>[2x]MHHH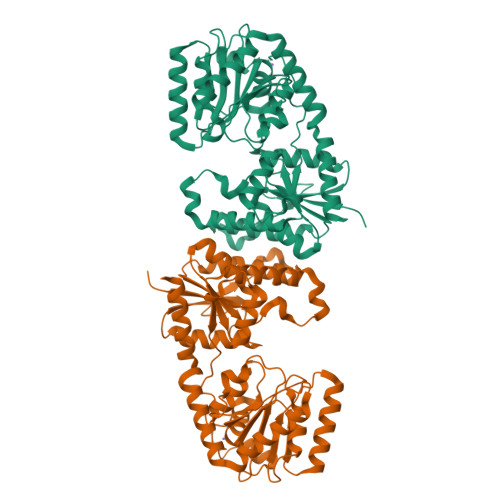HHHENLYFQGMRVAMMTREYPPEVYGGAGVHVTELVAQLRKLCDVDVHCMGAPRDGAYVAHPDPTLRGANAALTMLSADLNMVNNAEAATVVHSHTWYTGLAGHLASLLYGVPHVLTAHSLEPLRPWKAEQLGGGYQVSSWVERTAVEAADAVIAVSSGMRDDVLRTYPALDPDRVHVVRNGIDTTVWYPAEPGPDESVLAELGVDLNRPIVAFVGRITRQKGVAHLVAAAHRFAPDVQLVLCAGAPDTPQIAEEVSSAVQQLAQARTGVFWVREMLPTHKIREILSAATVFVCPSVYEPLGIVNLEAMACATAVVASDVGGIPEVVADGRTGLLVHYDANDTEAYEARLAEAVNSLVADPDRAREYGVAGRERCIEEFSWAHIAEQTLEIYRKVSA1-{4-[3-(2-METHOXY-BENZYLOXY)-PROPOXY]-PHENYL}-6-(1,2,,3,4-TETRAHYDRO-QUINOLIN-7-YLOXYMETHYL)-PIPERAZIN-2-ONE 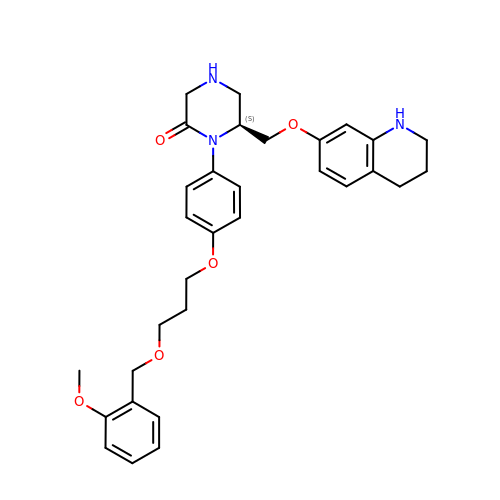| C31 H37 N3 O5 | JXFXZCANEQOOHW-SANMLTNESA-N>GSHMAHAGRTGYDNREIVMKYIHYKLSQRGYEWDAGDDVEENRTEAPEGTESEVVHLALRQAGDDFSRRYRGDFAEMSSQLHLTPFTARGRFATVVEELFRDGVNWGRIVAFFEFGGVMCVESVNREMSPLVDNIALWMTEYLNRH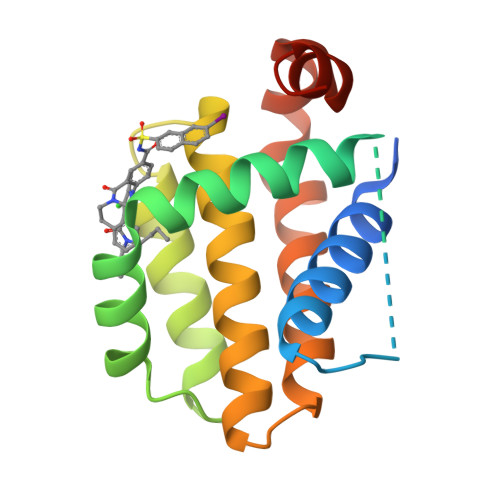LHTWIQDNGGWDAFVELYGPSMR[6x]> MVKLAFPRELRLLTPSQFTFVFQQPQRAGTPQITILGRLNSLGHPRIGLTVAKKNVRRAHERNRIKRLTRESFRLRQHELPAMDFVVVAKKGVADLDNRALSEALEKLWRRHCRLARGS

Ribonuclease P (RNase P) is an endonuclease whose primary role is to remove diverse 5′ leader sequences from precursor tRNAs (ptRNAs). Bacterial RNase P consists of a ~400 nucleotide P RNA and a single protein (rnpA, ~120 amino acids). RNase P recognizes the shape of the stacked acceptor and T-stems which span the two domains that together form a molecular ruler. In bacterial RNase P the 3′ RCCA of ptRNA pairs with a loop or internal bulge in the C-domain (L15), while a conserved adenosine in the catalytic core contacts an optimal U(−1) flanking the cleavage site 5′ to N(1).

To better understand how unwinding occurs and delineate the structural basis for such plasticity, we used cryo-electron microscopy (cryoEM) single particle analysis (SPA) to determine the structures of holoenzyme and ES* complexes formed with ptRNA_GG and ptRNA_AU. The ptRNA_AU substrate has the optimal consensus leader while ptRNA_GG contains the slowest dinucleotide sequence at N(−1)N(−2). We measured a 13-fold lower kcat/Km for ptRNA_GG compared to ptRNA_AU in single substrate assays. In contrast approximately half of the bound ptRNA_GG dissociated rapidly while the remainder was still bound. In both ptRNA_AU and ptRNA_GG bound complexes, the 5′ leader is positioned with the correct phosphodiester bond placed in the active site, while the 3′ RCCA is trapped in the L15 internal bulge loop of RNase P. In contrast, a larger nucleobase at the N(−1) position of ptRNA leader sequence, as in the case of ptRNA_GG-bound complex, sits in the cavity between J5/15 and J18/2 of RNase P thereby forcing the A248 nucleobase to tilt away from the leader sequence and stack with C73 of ptRNA. As such, RNase P uses a rotating glycosidic bond of A248 to help sculpt a flexible binding site to accommodate different nucleotides at N(−1), all while maintaining the correct active site geometry for the transition state. The N(−2) position of the ptRNA leader stacks with A333 of RNase P in both the ptRNA_AU and ptRNA_GG complexes. Notably, the distribution of the three classes identifies a significantly larger proportion of ptRNA-bound RNase P for the ptRNA_AU (~80% ES* complex) over ptRNA_GG (~46% ES* complex) dataset.> AAAAAAMTMMDMNFKYCHKIMKKHSKSFSYAFDLLPEDQRKAVWAIYAVCRKIDDSIDVYGDIQFLNQIKEDIQSIEKYPYEYHHFQSDRRIMMALQHVAQHKNIAFQSFYNLIDTVYKDQHFTMFETDAELFGYCYGVAGTVGEVLTPILSDHETHQTYDVARRLGESLQLINILRDVGEDFENERIYFSKQRLKQYEVDIAEVYQNGVNNHYIDLWEYYAAIAEKDFRDVMDQIKVFSIEAQPIIELAARIYIEILDEVRQANYTLHERVFVEKRKKA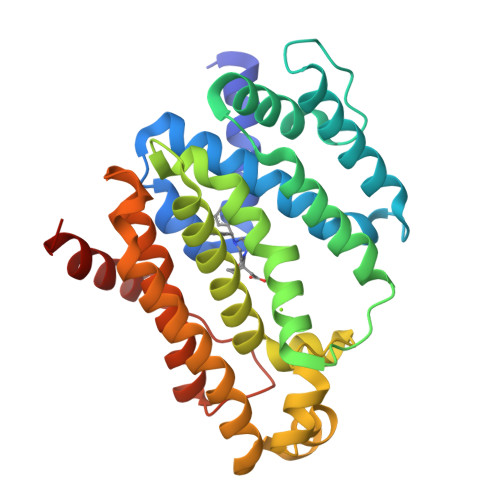KLFHEINSKYHRI> MSHHHHHHSGSGSGEKEEAEEVVKEALKELKKLFEEQKKVNEEAAKELEETAKDEKVLLAARFAVEASRIANKASFDLSKFAADAAAAAVEAGADIERVKEVLEKAIEAQKEAAKFSKKVLEEAAAAAALAERGEITEEDVARFVVELALELLKALFEMQRFVNELAAELLEVVAKDEKVLLAARFAVEASKIANEASFELSRFAAEAAAAAVEAGADI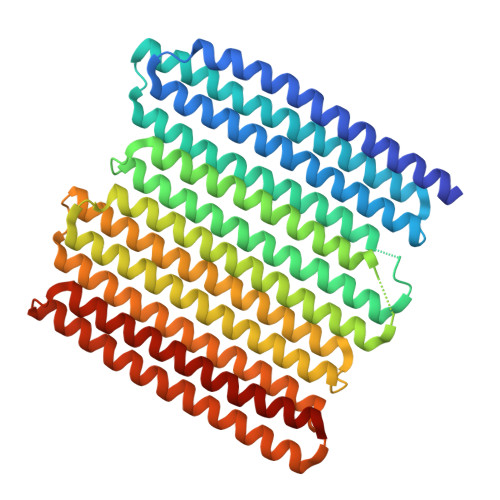ERVAEVLIKAIEAQAEAAKFSAEVLLKAAAAAALAERGEITEEDVARFVVELALELLRALFEMQRFVNELAAELLEVVAKDEKVLLAARFAVEASEIANKASFDLSKFAADAARAAVEAGADIERVAEVLIEAIKAQAEAAKFSAEVLLKAAAAAALAERGEITEKDVARFVVELALELLEALFEMQRFVNELAAALLEVVAKDEEVLEKARKAVEDSKRENEASFEESRKAAEAAAAAVEAGADIDEVAKELIEAIKEQAEAAKESAKKLLEAAAEAALAERGEIT2-[({4-[(3R,5S)-3,5-dimethylpiperidin-1-yl]-3-phenoxyphenyl}carbonyl)amino]benzoic 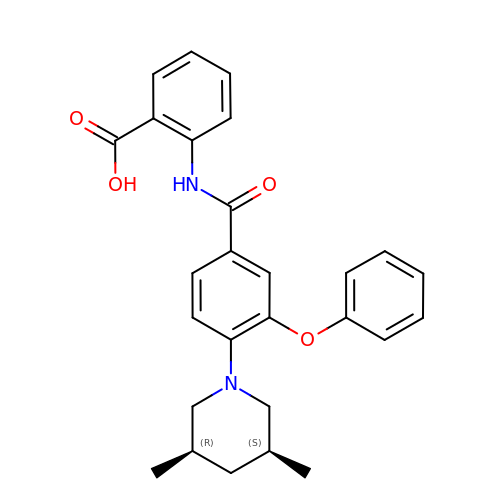acid | C27 H28 N2 O4 | YMZMFFRGSWCLPY-KDURUIRLSA-N> MAILKAQHLAKSYKKRKVVSDVSLQVESGQIVGLLGPNGAGKTTSFYMIVGLVARDEGTI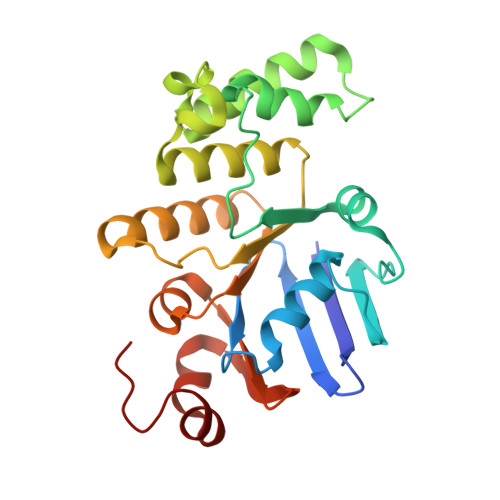TIDDNDISILPMHSRSRMGIGYLPQEASIFRKLSVEDNIMAVLQTREELTHEERQDKLEDLLEEFHIQHIRKSAGMALSGGERRRVEIARALAANPQFILLDQPFAGVDPISVIDIKKIIEHLRDRGLGVLITDHNVRETLDVCEKAYIVSQGRLIAEGTPQDVLNNEQVKQVYLGEQFRL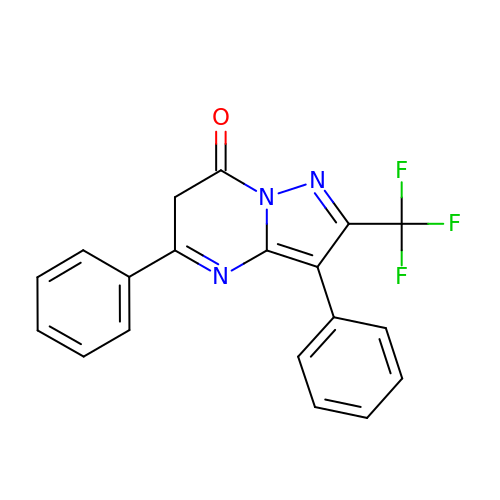3,5-diphenyl-2-(trifluoromethyl)-6~{H}-pyrazolo[1,5-a]pyrimidin-7-one | C19 H12 F3 N3 O | QLWOIKQIMHVRGX-UHFFFAOYSA-N> ADGRSTRYWDCCKPSCGWAKKAPVNQPVFSCNANFQRITDFDAKSGCEPGGVA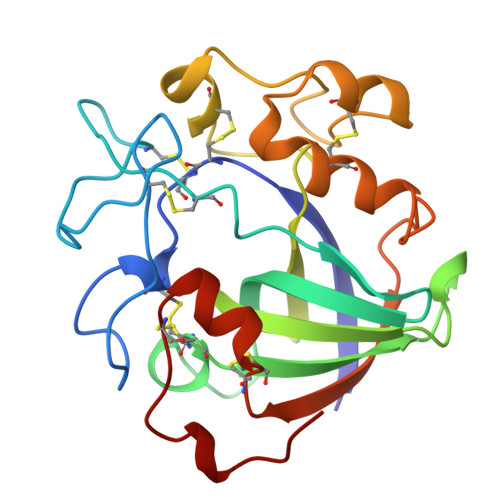YSCADQTPWAVNDDFALGFAATSIAGSNEAGWCCACYELTFTSGPVAGKKMVVQSTSTGGDLGSNHFDLNIPGGGVGIFDGCTPQFGGLPGQRYGGISSRNECDRFPDALKPGCYWRFDWFKNADNPSFSFRQVQCPAELVARTGCRRNDDGNFPAV> MHHHHHHHHENLYFQGGSSTAGDPT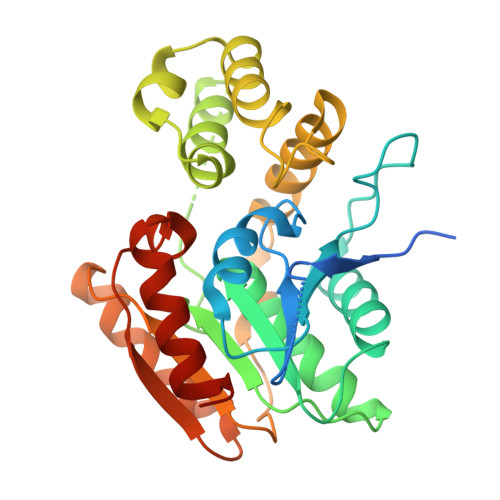AKLVRLNPRGGDGPGIVFAPPAGGTVLGYIELARHLKGFGEIHGVEAPGLGAGETPVYPSFEEMVQFCSDSAAGVAGDGVYIGGHSLGGHIAFYLATMLLDRGIRPKGLIILDTPPRLGDIPVADADLTEEETKVFILAMGIGGMLDQDRDALKDLPYEEAKQLLLDRAKNDPRVSAFLSEDYLDRFLRLQMHQLMYSRDVVLPQRKLDIPIHVFRTKNHAPEVARLFSAWENYAAGEVTFVDIPGDHATMLRAPHVSEVAQLLDRHCGLPSDDGPRG>MLSVGATTTATRLTGWGRTAPSVANVLRTPDAEMIVKAVARVAESGGGRGAIARGLGRSYGDNAQNGGGLVIDMTPLNTIHSIDADTKLVDIDAGVNLDQLMKAALPFGLWVPVLPGTRQVTVGGAIACDIHGKNHHSAGSFGNHVRSMDLLTADGEIRHLTPTGEDAELFWATVGGNGLTGIIMRATIEMTPTSTAYFIADGDVTASLDETIALHSDGSEARYTYSSAWFDAISAPPKLGRAAVSRGRLATVEQLPAKLRSEPLKFDAPQLLTLPDVFPNGLANKYTFGPIGELWYRKSGTYRGKVQNLTQFYHPLDMFGEWNRAYGPAGFLQYQFVIPTEAVDEFKKIIGVIQASGHYSFLNVFKLFGPRNQAPLSFPIPGWNICVDFPIKDGLGKFVSE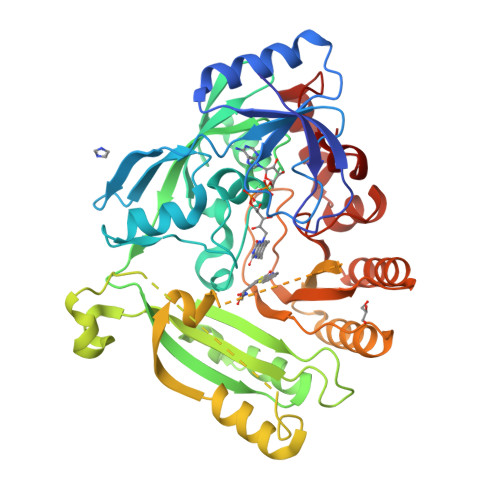LDRRVLEFGGRLYTAKDSRTTAETFHAMYPRVDEWISVRRKVDPLRVFASDMARRLELL[2x]> MKHQHQHQHQHQHQQPLQEEEQAHATSLPPRASSPPQILPQLSPEQLGMIEKLVAAQQQCNRRSFSDRLRVTPWPMAPDPHSREARQQRFAHFTELAIVSVQEIVDFAKQLPGFLQLSREDQIALLKTSAIEVMLLETSRRYNPG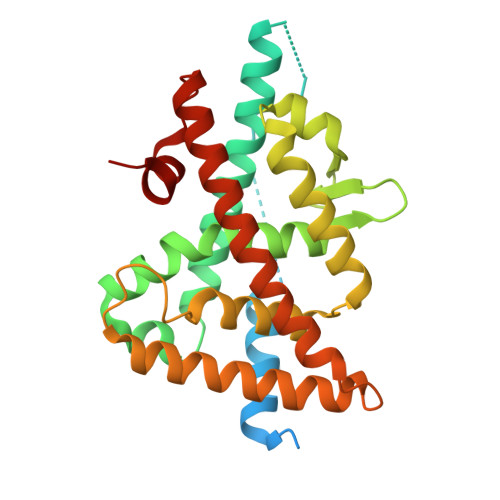SESITFLKDFSYNREDFAKAGLQVEFINPIFEFSRAMNELQLNDAEFALLIAISIFSADRPNVQDQLQVERLQHTYVEALHAYVSIHHPHDRLMFPRMLMKLVSLRTLSSVHSEQVFALRLQDKKLPPLLSEIWDVHE> MGSSHHHHHHSSGLVPRGSHMTTTISADQVNQIIYNLHHDPFEILGCHLLEEGKNTKKWVVRAYLPKAEAAWVIRPTERKEDPMNSVHHPNFFEC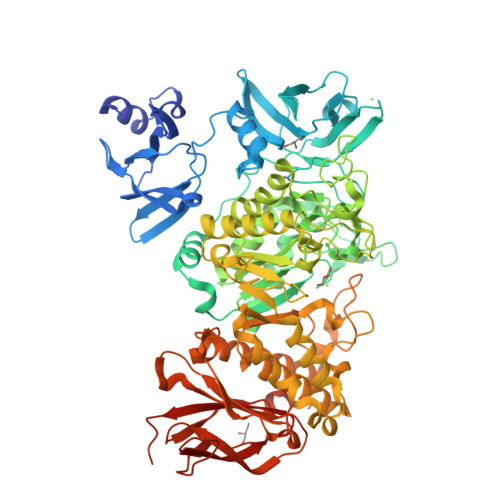IIETPELNHYQLKVKEGEHEKVIYDPYAFSSPYLTDEDIYLFSEGNHHRIYEKLGAHVGEINGVKGVYFAVWAPNARNVSVIGDFNNWDGREHQMRKRNYTIWELFVPEIGSGTVYKYEIKNSEGHIYEKSDPYGFYREVRPNTASIVVDIDNIYQWHDEEWLEKRRNSDPLKQPVSVYEVHLGSWLHGSSAEKMPLLNGEADPVIVSEWNPGARFLSYYELAEKLIPYVKDMGYTHIELLPIAEHPFDGSWGYQVTGFYSPTSRFGRPEDFMYFVDKCHENGIGVILDWVPGHFPKDSHGLAYFDGTHLYEHADPRIGEHKEWGTLVFNYGRHEVRNFLVANVLFWFDKYHVDGIRVDAVASMLYRNYLRKEGEWIANEYGGDEHIEAVSFIREVNTLLFEYFPGILSIAEESTEWEKVSRPVYDGGLGFNLKWDMGWMHDMLDYFNIDPYFRQYHQNNVTFSMAYYYNENFMLALSHDEIVHGKSNMLGKMPGDEWQKYANVRALFTYMYTHPGKKTMFMSMEFGQWSEWNVWGDLEWHLLQYEPHQQLKQFFTDLNALYQQEPALYTHDFEYHGFEWIDCNDNTHSVVSFLRRSDDPNDSLVVVCNFTPQPHSHYRIGVPEAGYYVELFNSDAKQYGGSNMGNLGGKWADEWSFHNKPYSLDLCLPPLAVLILKLDPTKVPEGTTIKEIAADEEE> MHDANRFGGRTAYLREIGPIDHKKKGRLFKRDL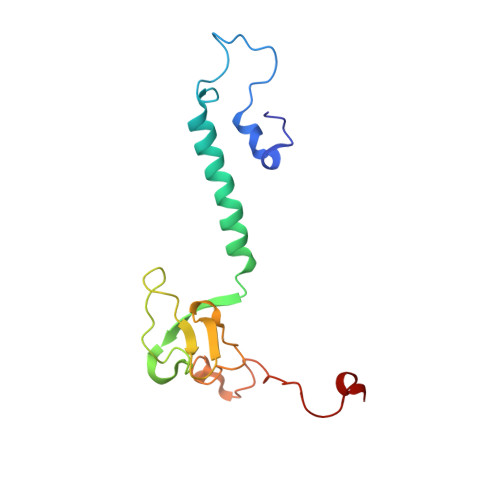PTLQFNVDVWCAQQTLRKQWKGRDWDVVEMPFEMAPKELQRVVPEKYTDVPIMTDPARHDYMNIRRKVFDREDMQDALFASGGAGQSPYPAIQRVDKAAMTLDKYL>GHMEVTLIVFHAGSLSVPFQEVEKEFSEYAERNLGI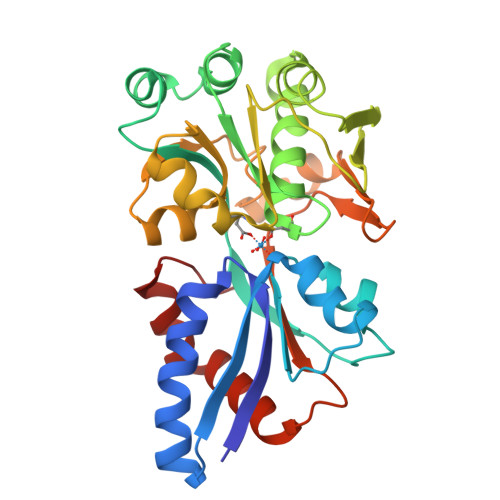KVSFQDEASGSVMAVRKVTDLGRKADVIGVADYTLIPQLLIPNYTDFYVLFATNEIVIAFTDKSRYVEEMKSNPDKWYEILAREDVRFGFSDPNQDPCGYRSLMVIKLADLYYGKEIFKELIEENTNIYSNGTQIYAPKEITVNPGKIVIRPKETDLLGLVESGSIDYIFIYKSVAKQHNLSYITLPSEINLGDFSKEKFYGQISITLGSTGKTIKAKPIVYGVTVLKDAPNREVAIEFLRYLLSENGKRIFEKNHQDFL[2x]> GSPGIPMVAAHAAHSQSSAEWIACLDKRPLERSSEDVDIIFTRLKGVKAFEKFHPNLLRQICLCGYYENLEKGITLFRQGDIGTNWYAVLAGSLDVKVSETSSHQDAVTICTLGIGTAFGESILDNTPRHATIVTRESSELLRIEQEDFKALWEKYRQYMAGLLAPPYGVMETGSNNDRIPDKENVPSEKILRAGKILRIAILSRAPHMIRDRKYHLKTYRQCCVGTELVDWMIQQTSCVHSRTQAVGMWQVLLEDGVLNHVDQERHFQDKYLFYRFLDDEREDAPLPTEEEKKECDEELQDTMLLLSQMGPDAHMRMILRKPPGQRTVDDLEIIYDELLHIKALSHLSTTVKRELAGVLIFESHAKGGTVLFNQGEEGTSWYIILKGSVNVVIYGKGVVCTLHEGDDFGKLALVNDAPRAASIVLREDNCHFLRVDKEDFNRILRDVEANTVRLKEHDQDVLVLEKVPAGNRAANQGNSQPQQKYTVMSGTPEKILEHFLETIRLEPSLNEATDSVLNDFVMMHCVFMPNTQLCPALVAHYHAQPSQGTEQERMDYALNNKRRVIRLVLQWAAMYGDLLQEDDVAMAFLEEFYVSVSDDARMMAAFKEQLPELEKIVKQISEDAKAPQKKHKVLLQQFNTGDERAQKRQPIRGSDE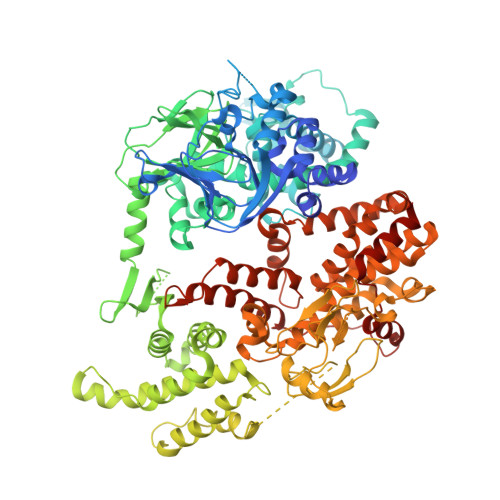VLFKVYCIDHTYTTIRVPVAASVKEVISAVADKLGSGEGLIIVKMNSGGEKVVLKSNDVSVFTTLTINGRLFACPREQFDSLTPLPEQEGPTTGTVGTFELMSSKDLAYQMTTYDWELFNCVHELELIYHTFGRHNFKKTTANLDLFLRRFNEIQFWVVTEVCLCSQLSKRVQLLKKFIKIAAHCKEYKNLNSFFAIVMGLSNVAVSRLALTWEKLPSKFKKFYAEFESLMDPSRNHRAYRLTAAKLEPPLIPFMPLLIKDMTFTHEGNKTFIDNLVNFEKMRMIANTARTVRYYRSQPFNPDAAQANKNHQDVRSYVRQLNVIDNQRTLSQMSHRLEPRRP> AYFQSMSRLPVIVGFGGYNAAGRSSFHHGFRRMVIESMDPQARQETLAGLAVMMKLVKAEGGRYLAEDGTPLSPEDIERRYAERIFASTLVRRIEPQYLDPDAVHWHKVLELSPAEGQALTFKASPKQLPEPLPANWSIAPAEDGEVLVSIHERCEFKVDSY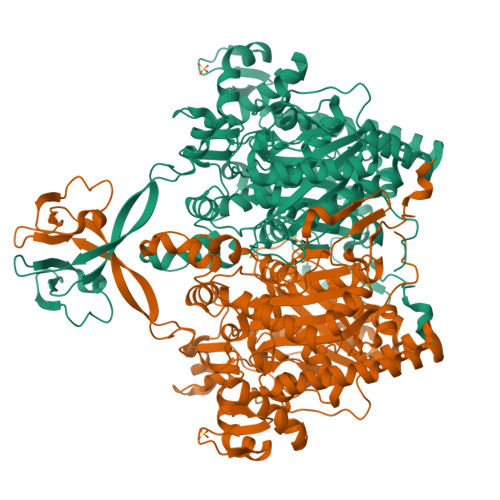RALTVKSAGQLPTGFEPGELYNSRFHPRGLQMSVVAATDAIRSTGIDWKTIVDNVQPDEIAVFSGSIMSQLDDNGFGGLMQSRLKGHRVSAKQLPLGFNSMPTDFINAYVLGSVGMTGSITGACATFLYNLQKGIDVITSGQARVVIVGNSEAPILPECIEGYSAMGALATEEGLRLIEGRDDVDFRRASRPFGENCGFTLAESSQYVVLMDDELALRLGADIHGAVTDVFINADGFKKSISAPGPGNYLTVAKAVASAVQIVGLDTVRHASFVHAHGSSTPANRVTESEILDRVASAFGIDGWPVTAVKAYVGHSLATASADQLISALGTFKYGILPGIKTIDKVADDVHQQRLSISNRDMRQDKPLEVCFINSKGFGGNNASGVVLSPRIAEKMLRKRHGQAAFAAYVEKREQTRAAARAYDQRALQGDLEIIYNFGQDLIDEHAIEVSAEQVTVPGFSQPLVYKKDARFSDMLD>[2x]MFENITATTADPILGLADLFRADERPGKIDLGIGVYKDETGKTPVLTSVKKAEQYLLENETTKNYLGIDGIPEFGRCTQELLFGKGSALINDKRARTAQTPGGSGALRVAADFLAKNTSVKRVWVSNPSWPNHKSVFNSAGLEVREYAYYDAENHTLDFDALINSLNEAQAGDVVLFHGCCHNPTGIDPTLEQWQTLAQLSVEKGWLPLFDFAYQGFAR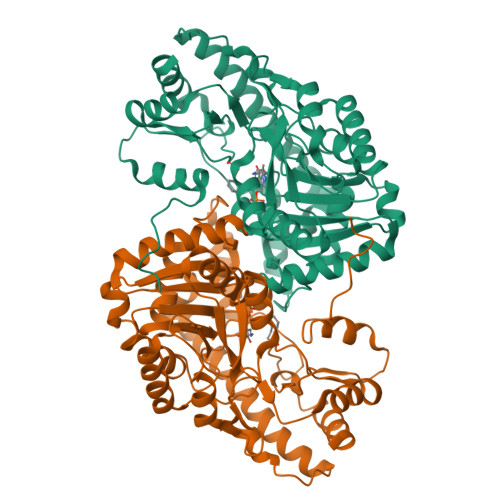GLEEDAEGLRAFAAMHKELIVASSYSKNFALYNERVGACTLVAADSETVDRAFGQMKAAIRDNYSSPPAHGASVVATILSNDALRAIWEQELTDMRQRIQRMRQLFVNTLQEKGANRDFSFIIKQNGMFSFSGLTKEQVLRLREEFGVYAVASGRVNVAGMTPDNMAPLCEAIVAVL6-cyano-4-[[(1R)-1-(4-methylphenyl)ethyl]amino]quinoline-3-carboxamide 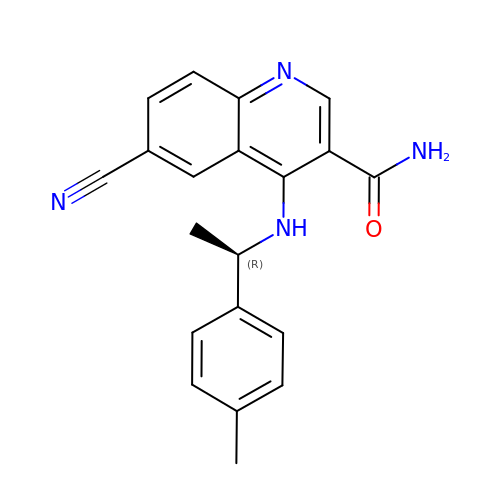| C20 H18 N4 O | STFKVULAQFVZBR-CYBMUJFWSA-N> LSVDPATCPIVPGQEMIIEISKGR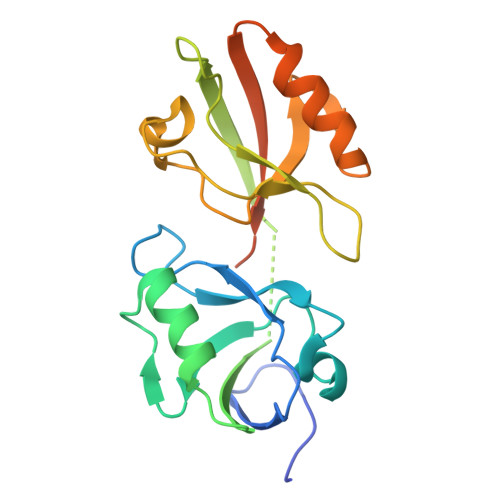SGLGLSIVGGKDTPLNAIVIHEVYEEGAAARDGRLWAGDQILEVNGVDLRNSSHEEAITALRQTPQKVRLVVYRDEAHYRDEENLEIFPVDLQKKAGRGLGLSIVGKRNGSGVFISDIVKGGAADLDGRLIQGDQILSVNGEDMRNASQETVATILKCAQGLVQLEIGRLRAGSWTSARTTGGGSGGGGSGG> RVPPPPPCCHPRLSLHRPALEDLLLGSEANLTCTLTGLRDASGATFTWTPSSGKSAVQGPPERDLCGCYSVSSVLPGSAQPWNHGETFTCTAAHPELKTPLTATLSKSGNTFRPEVHLLPPPSEELALNELVTLT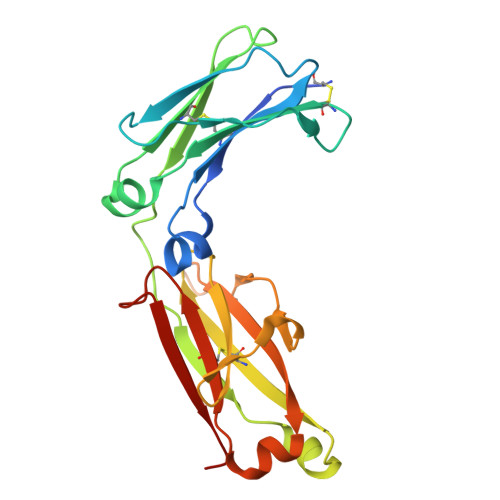CLARGFSPKDVLVRWLQGSQELPREKYVTTASRQEPSQGTTTFAVTSLLRVAAEDWKKGDTFSCMVGHEALPLAFTQKTIDRLAG>[4x]MADKTTETVPIPGPPGLPLVGNALAFDSELPLRTFQEFAEEYGEIYRLTLPTGTTLVVSSQALVHELCDDKRFKKPVAAALAEVRNGVNDGLFTAREEEPNWGIAHRILMPAFGPASIQGMFTEMHEIASQLALKWARHGPDTPIFVTDDFTRLTLDTLALCTMNFRFNSYYHDELHPFINAMGNFLTESGARAMRPAITSIFHQ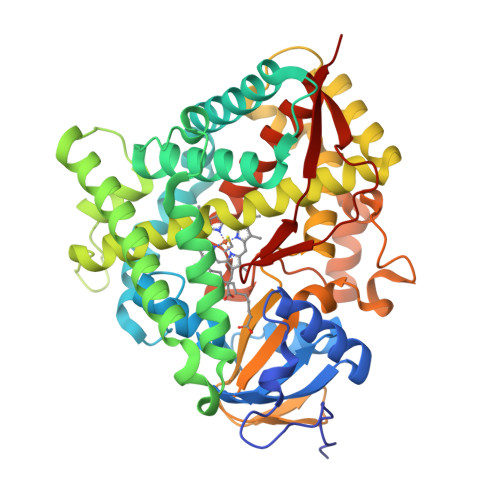AANRKYWEDIEVLRKTAQGVLDTRRKHPTNRKDLLSAMLDGVDAKTGQKLSDSSIIDNLITFLIAGHETTSGLLSFAFYLLIKHQDAYRKAQEEVDRVIGKGPIKVEHIKKLPYIAAVLRETLRLCPTIPIINRAAKQDEVIGGKYAVAKDQRLALLLAQSHLDPAVYGETAKQFIPERMLDENFERLNREYPDCWKPFGTGMRACIGRPFAWQEAVLVMAMLLQNFDFVLHDPYYELHYKQTLTTKPKDFYMRAILRD> EEDC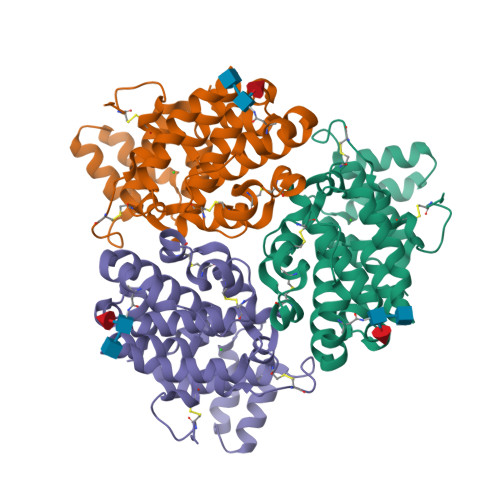WKNEELKEDCVGPLIAPKDCTDKDHKTYLSEASLLATAKKITQVDAENVEILGKTMESAIRVIERQKTYHRMHLLEAVFLNKHCDYYKMFEHNSGYSQVKWRMMIKTQHFDICALQANSPFCAQCIADNSCAQGSWEFDTHMNSTYSSKVDNFKHDFSLFLRIFEAAFPGTAYVHLLTNIKEKKPYQAVSMIEKIKKKFPNNKLLIGYLDFGKYLLGLSHASTYELQQRQLDKLYQPTELGGWSHPQFEK>[4x]SGSGSTAEPDL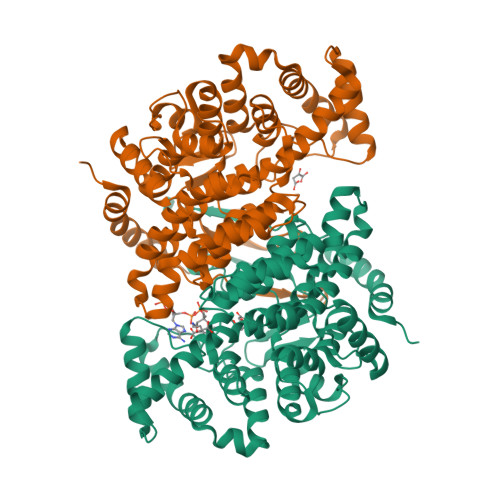KTALKAVIPAKRELFKQVKERSDEVIGEVKVANVIGGMRGLKSMLWEGSVLDPEEGIRFHGKTIKDCQKELPKGTSGTEMLPEAMFWLLLTGQVPSTNQVRAFSRELAEQSHLPQHILDLIKSFPRSMHPMTQLSIAVAALNTESKFAKAYEKGLSKADYWEPTFDDSISLLAKIPRVAALVFRPDEVDQVGTQALDASQDWSYNFAELLGKGGKENQDFHDLLRLYLALHGDHEGGNVSAHATHLVGSALSDPFLSYSAGLLGLAGPLHGLAAQEVLRWILAMQDKIGTKFTDDDVRNYLWDTLKSGRVVPGYGHGVLRKPDPRFQALMDFAATRPDVLANPVFQLVKKNSEIAPAVLTEHGKTKNPHPNVDAASGVLFYHYGFQQPLYYTVTFGVSRALGPLVQLIWDRALGLPIERPKSINLLGLKK> SFKYESAVQYRPAPDSYLNPCPQAGRIVKETYTGINGTKSLNVYLPYGYDPNKKYNIFYLMHGGGENENTIFSNDVKLQNILDHAIMNGELEPLIVVTPTFNGGNCTAQNFYQEFRQNVIPFVESKYSTYAESTTPQGIAASRMHRGFGGFSMGGLTTWYVMVNCLDYVAYFMPLSGDYWYGNSPQDKANSIAEAINRSGLSKREYFVFAATGSEDIAYANMNPQIEAMKALPHFDYTSDFSKGNFYFLVAPGATHWWGYVRHYIYDALPYFFHE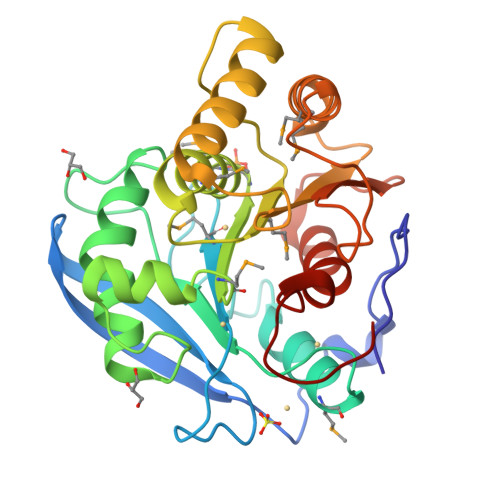LEHHHHHH3-PROPYL-5-(3-PYRIDYL)-1H-PYRAZIN-2-ONE 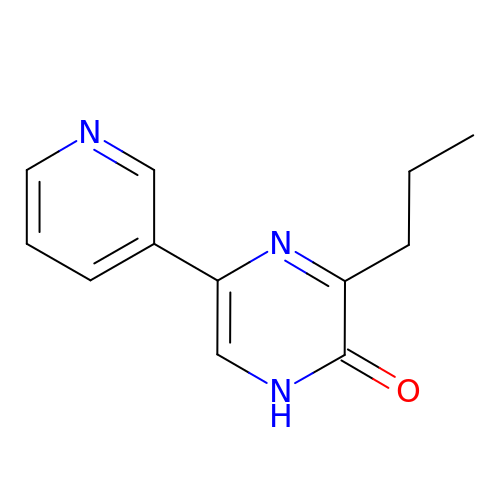| C12 H13 N3 O | ZKLHKFWUNCAKLE-UHFFFAOYSA-N>DDHSELLVNTKSGKVMGTRVPVLSSHISAFLGIPFAEPPVGNMRFRRPEPKKPWSGVWNASTYPNNCQQYVDEQFPGFSGSEMWNPNREMSEDCLYLNIWVPSPRPKSTTVMVWIYGGGFYSGSSTLDVYNGKYLAYTEEVVLVSLSYRVGAFGFLALHGSQEAPGNVGLLDQRMALQWVHDNIQFFGGDPKTVTIFGESAGGASVGMHILSPGSRDLFRRAILQSGSPNCPWASVSVAEGRRRAVELGRNLNCNLNSDEELIHCLREKKPQELIDVEWNVLPFDSIFRFSFVPVIDGEFFPTSLESMLNSGNFKKTQILLGVNKDEGSFFLLYGAPGFSKDSESKISREDFMSGVKLSVPHANDLGLDAVTLQYTDWMDDNNGIKNRDGLDDIVGDHNVICPLMHFVNKYTKFGNGTYLYFFNHRASNLVWPEWMGVIHGYEIEFVFGLPLVKELNYTAEEEALSRRIMHYWATFAKTGNPNEPHSQESKWPLFTTKEQKFIDLNTEPMKVHQRLRVQMCVFWNQFLPKLLNATACDGELSSSGTSSSKGIIFYVLFSILYLIF[2x]

Diagnostic testing and symptomatic treatment of myasthenia gravis are based on restoration of cholinergic transmission at the neuromuscular junction by means of peripherally-acting inhibitors of acetylcholinesterase (AChE), the enzyme responsible for the hydrolysis of the neurotransmitter acetylcholine at the synapse. Inhibition of acetylcholine breakdown renders the neurotransmitter more available for nicotinic AChR stimulation, which alleviates muscle weakness by improving neuromuscular transmission. In this study, we explored two different approaches to accessing more polar derivatives of tacrine, 6-chlorotacrine, and huprine Y, which may serve as new peripherally-acting AChEIs of potential value for treatment of myasthenia gravis. Furthermore, the three-dimensional structures of complexes of several of these compounds with Torpedo californica AChE (TcAChE) were also solved, in order to shed light on their mechanism of action.

In the crystal structure of TcAChE complexed with the 6-chlorotacrine-based quinolinium derivative 5, we found three molecules of 5 bound to each of the two monomers present in the asymmetric unit. While the conjugated system of the molecule is sandwiched between Trp84 and Phe330, making a π-stacking interaction with Trp84, the orientation of the chlorine atom is quite unusual. In the TcAChE/5 complex, the chlorine atom faces the opposite side of the gorge, pointing towards the main-chain of residues 116–118. In this orientation, the nitrogen of the exocyclic amino group H-bonds to the carbonyl of catalytic His440 (2.73 Å), and the methyl group points towards the entrance of the gorge. The loss of the important interactions of the chlorine atom in the above-mentioned hydrophobic pocket is most probably at the origin of the 300-fold drop of potency when compared to 6-chlorotacrine. We decided, therefore, to model a second, minor, orientation in the active site of TcAChE. In this orientation, the nitrogen atom of the exocyclic amino group is H-bonded to water molecules, while the methyl group faces the main chain of catalytic Ser200 (2.74 Å). This close contact of the methyl group with the protein is probably the reason that this conformation is poorly populated. Other large electron density blobs in the mFo-DFc maps indicated the presence of a second copy of 5 at the PAS. 5 was modeled, making a π–π stacking with Trp279, but in two alternate conformations, with the Cl atom pointing either into or out of the gorge.> GNKICQFKLVLLGESLVGKSSLVLRFVKGQFHEFQESTIGAAFLTQTVCLDDTTVKFEIWDTAGQERYHSLAPMYYRGAQAAIVVYDITNEESFARAKN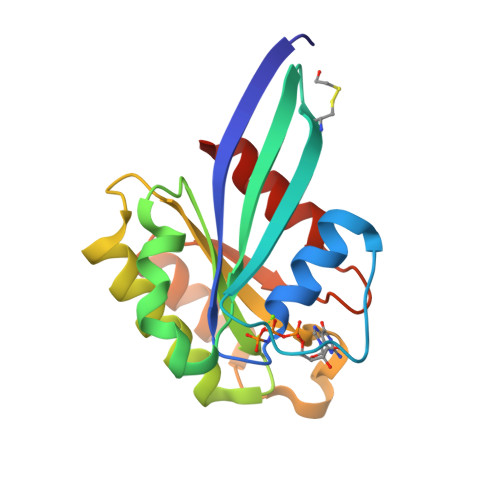WVKELQRQASPNIVIALSGNKADLANKRAVDFQEAQSYADDNSLLFMETSAKTSMNVNEIFMAIAKKLPKN> MSQRITIDPVTRIQGHLRIDCEIENGVVSKAWASGTMWRGMEEIVKNRDPRDAWMIVQRICGVCTTTHALSSVRAAESALNIDVPVNAQYIRNIILAAHTTHDHIVHFYQLSALDWVDITSALQADPTKASEMLKGVSTWHLNSPEEFTKVQNKIKDLVASGQLGIFANGYWGHPAMKLPPEVNLIAVAHYLQALECQRDANRVVALLGGKTPHIQNLAVGGVANPINLDGLGVLNLERLMYIKSFIDKLSDFVEQVYKVDTAVIAAFYPEWLTRGKGAVNYLSVPEFPTDSKNGSFLFPGGYIENADLSSYRPITSHSDEYLIKGIQESAKHSWYKDEAPQAPWEGTTIPAYDGWSDDGKY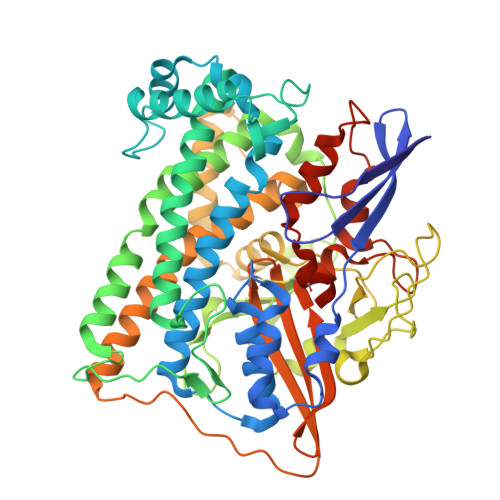SWVKSPTFYGKTVEVGPLANMLVKLAAGRESTQNKLNEIVAIYQKLTGNTLEVAQLHSTLGRIIGRTVHCCELQDILQNQYSALITNIGKGDHTTFVKPNIPATGEFKGVGFLEAPRGMLSHWMVIKDGIISNYQAVVPSTWNSGPRNFNDDVGPYEQSLVGTPVADPNKPLEVVRTIHSFDPCMACAVHVVDADGNEVVSVKVL>MELDGDQMISHRELWAKIANSINDINEQYLKVYEHAVSSYTQMYQDFSAVLSSLAGWISPGGNDGNSVKLQVNSLKKALEELKEKYKDKPLYPANNTVSQEQANKWLTELGGTIGKVSQKNGGYVVSINMTPIDNMLKSLDNLGGNGEVVLDNAKYQAWNAGFSAEDETMKNNLQTLVQKYSNANSIFDNLVKVLSSTISS[2x]

Like many Gram-negative pathogens, Shigella rely on their type three secretion system (T3SS) to inject effector proteins into eukaryotic host cells, driving both cellular invasion and evasion of host immune responses. Studies in Shigella have demonstrated that bile salts found in the small intestine (e.g., deoxycholate (DOC)) interact directly with the injectisome tip complex protein invasion plasmid antigen D (IpaD) to support interaction with the hydrophobic translocator protein IpaB and its stable recruitment to the maturing tip complex. In Shigella, IpaD resides at the extracellular tip of the injectisome where it functions as a “gatekeeper” that prevents unwanted protein secretion (leakage) through the injectisome prior to requisite activation events. Here, we uncover critical mechanistic details of the Shigella-specific DOC signaling process by describing the role of a π-helix secondary structure element within the T3SS tip protein invasion plasmid antigen D (IpaD).

A small number of groups, including our own, have crystallized IpaD and IpaD mutants and while some full-length IpaD structures have been solved, proteolytic cleavage of the N-terminal domain facilitates crystallization. Here, we mimicked the previously successful native proteolytic cleavage by engineering IpaDWT, IpaDΔQ148, and IpaDΔY149 to lack their N terminal 121 residues. These N-terminal truncation constructs expressed and purified well in E. coli and diffracting crystals of IpaDΔ1–121, WT and IpaDΔ1–121, ΔQ148 formed overnight by vapor diffusion. Careful consideration of the WT structure suggested that the localized i + 5 hydrogen bonding pattern of the π-helix results from the “insertion” of an amino acid into this region and that removing either the glutamine at position 148 or the tyrosine at position 149 would eliminate the π-helix and return it to a continuous i + 4 hydrogen bonding α-helix. Aligning the IpaDΔ1–121, WT and IpaDΔ1–121, ΔQ148 structures additionally shows that Y149 sterically prevents the F308 rotamer change in the WT π-helix structure. Notably, while very modest conformational changes are observed in the crystal structures as a result of DOC binding to either the IpaDΔ1–121, WT or IpaDΔ1–121, ΔQ148 structures, the removal of the π-helix in both the apo and bound conditions results in a lateral shift of the central helices relative to the WT structure, resulting in a 7 Å translation of the distal ends of the structures.> XSKSK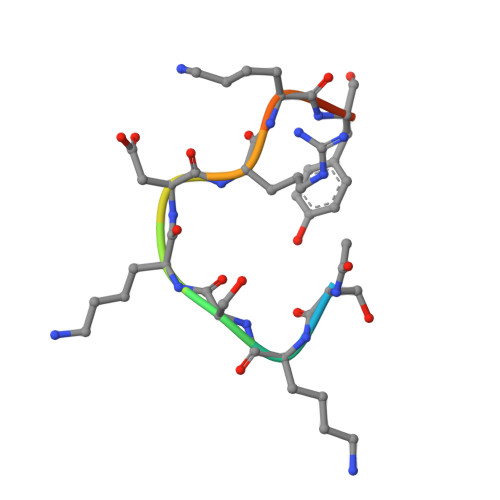DRKYTL>[8x]MAGNF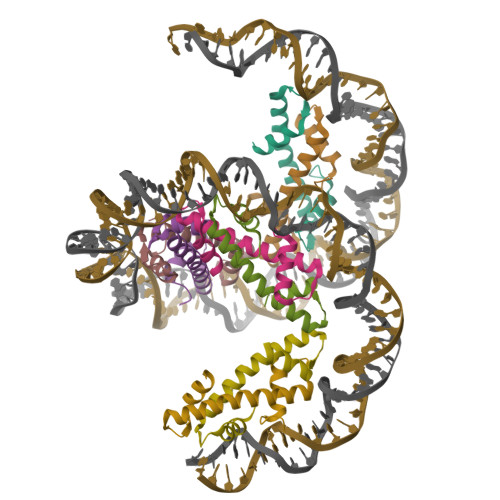ANARVEKLIRQAGAQRVSADAVDKMNEILTDWGKNIAKYAVEIARHSGRKTVKENDIKLAAQK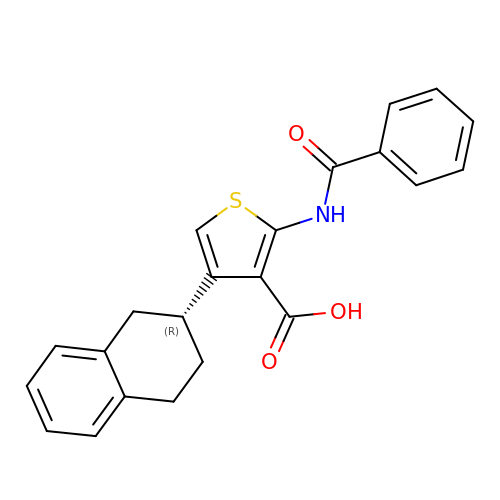2-benzamido-4-[(2~{R})-1,2,3,4-tetrahydronaphthalen-2-yl]thiophene-3-carboxylic acid | C22 H19 N O3 S | ITAWNUSVGMPVHR-QGZVFWFLSA-N>[2x]MTNVLIVEDEQAIRRFLRTALEGDGMRVFEAETLQRGLLEAA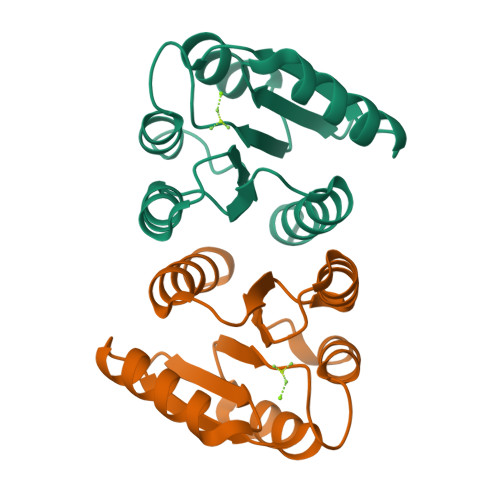TRKPDLIILDLGLPDGDGIEFIRDLRQWSAVPVIVLSARSEESDKIAALDAGADDYLSKPFGIGELQARLRVALRRHSQ>[2x]AGSMIRTMLQGKLHRVKVTHADLHYEG;>[2x]SCAIDQDFLDAAGILENEAIDIWNVTNGKRFSTYAIAAERGSRIISVNGAAAHCASVGDIVIIASFVTMPDEEARTWRPNVAYFEGDNEMKRTA

ADC catalyzes the oxidative decarboxylation of l-aspartate to yield β-alanine. β-Alanine is required for the biosynthesis of pantothenate (vitamin B5)18 which is then further converted to the important metabolic cofactor, Coenzyme A.17 ADC contains a covalently linked protein-derived pyruvoyl cofactor which forms a Schiff base with the substrate to initiate the decarboxylation reaction. This protein-derived cofactor is formed via the post-translational cleavage of the ADC zymogen protein backbone into α and β chains, resulting in the formation of a new C-terminus on the α chain and a N-terminal pyruvoyl cofactor on the β chain. The α C-terminus is extremely flexible, and the initial binding of the substrate is associated with its rearrangement to close over the active site. This conformational rearrangement is believed to play a role in determining the overall rate of catalysis.21d-serine is an inhibitor of ADC that, like the substrate l-aspartate binds in the enzyme active site.

We have determined the structure of ADC in the presence of the d-serined-serine ligand using X-ray diffraction. As in the apo-ADC structure, the liganded ADC tetramer is formed by a crystallographic two-fold, with two ADC monomers in the asymmetric units. As in the apo structure, a fraction of mis-processed ADC is present, where the backbone of the zymogen is cleaved, but the β subunit has an N-terminal serine instead of a pyruvate. This mis-processed form is present at ≈40% occupancy. The d-serine molecule adopts two conformations in both subunits of the asymmetric unit. One conformer (60% occupancy) forms hydrogen bonds with the main chain of ALA-75, the side-chains of ARG-54 and THR-57, and the pyruvoyl carbonyl (ESI†) adopting a similar binding conformation to the native substrate l-aspartate. The second conformer (40% occupancy) forms hydrogen bonds with the side-chains of LYS-9 and TYR-58 (ESI†) and with the nitrogen atom of the mis-processed β N-terminal SER-25. The degree of “openness” is not the same in the two ADC subunits of the asymmetric unit. There is a significant change in the conformation of the α C-terminal loop of chain A (subunit 1) which shows a displacement of 4.3 Å of the Cα of GLU-23 from its position in the apo structure and a clear change in the conformation of its side-chain (bottom). However, for chain D (subunit 2), the structural change is relatively small with a Cα–Cα distance of only 0.8 Å for the same residue, although d-serine is bound in both subunits (top).> MFGRLVLKQTRRTLFNPVLKNTFCIYQAYQNPLRHINTGHNPNNVYEDIVMLGDYPVQNRTHDKVISQTYVPAIANIAFTHLSKKYPQAGLKVDQLNTLKEKT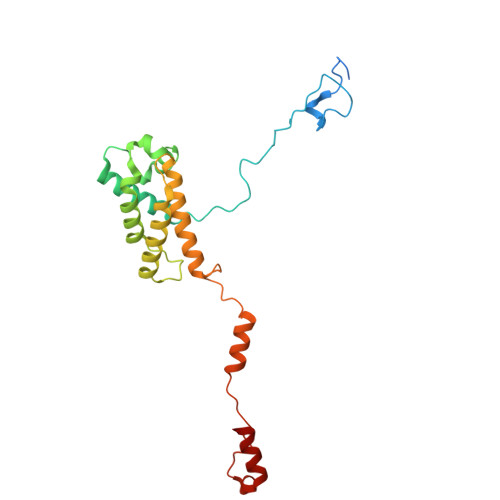WNDLGVNIEHEKQEILVELSEQIFVKESKLRWVHEQRQRLAHTTYVFSGLEFQNVKVGFFIDSYNFLLQELAHRSNLYQSKDIVGEKSFHEKHLEQQTAPYSGVKSLEEPVSQNKSFINSLMRAIHNH> PRGGKIVVTVRLWDEPIAAAYRQSFAAFTRSHPDIEVRTNLVAYSTYFETLRTDVAGGSADDIFWLSNAYFAAYADSGRLMKIQTDAADWEPAVVDQFTRSGVLWGVPQLTDAGIAVFYNADLLAAAGVDPTQVDNLRWSRGDDDTLRPMLARLTVDADGRTANTPGFDARRVRQWGYNAANDPQAIYLNYIGSAGGVFQRD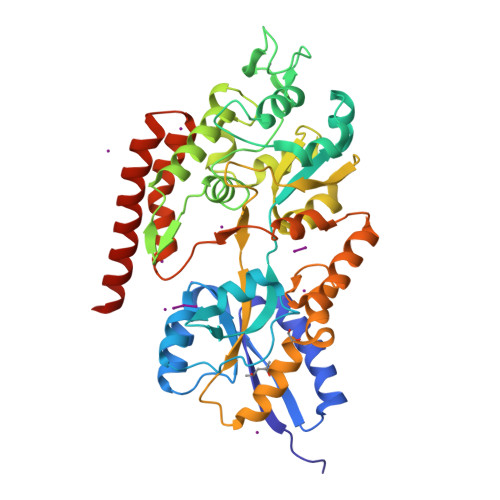GKFAFDNPGAIEAFRYLVGLINDDHVAPPASDTNDNGDFSRNQFLAGKMALFQSGTYSLAPVARDALFHWGVAMLPAGPAGRVSVTNGIAAAGNSASKHPDAVRQVLAWMGSTEGNSYLGRHGAAIPAVLSAQPVYFDYWSARGVDVTPFFAVLNGPRIAAPGGAGFAAGQQALEPYFDEMFLGRGDVTTTLRQAQAAANAATQRKLAAALEHHHHHH> HMPRVLVTGALGQIGTDLSLALRDKFGAD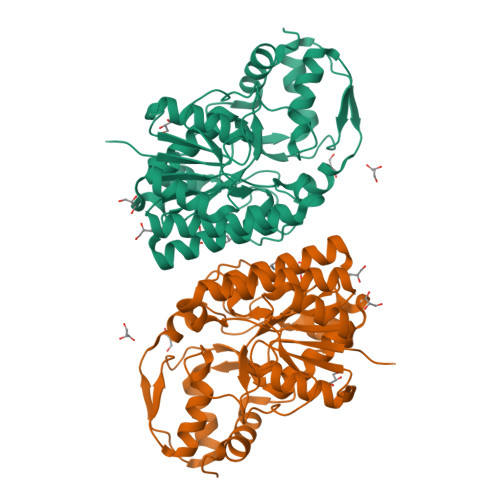SVLVSDVVEPGAKHPLAGLKGVEKLDCLDSNGFEKLVKEFKPTWMYHLPAIMSVRGEAEPDLAMDINVNTTRYALELARKYNIRIFIPSTIAAFGDKCGKTMTKDDTIMNPSTVYGVTKVYTELLGTWYRQKYGVDFRSVRLPGIISAATLPGGGATDYAIHMYHSALLQKKCVCPVLPYESLPMMYMPDTLNSLVKIMEAPLEKLTRTVYNITGFSFSPSELRFSIERCTDRTIEVEYVEGPAQKIANSWPDSLDDSNARNDWGHQVKYDIDMMSEDMLRQIPILHGLPSL> AKIIFIEHNGTRHEVEAKPGLTVMEAARDNGVPGIDADCGGACACSTCHAYVDPAWVDKLPKALPTET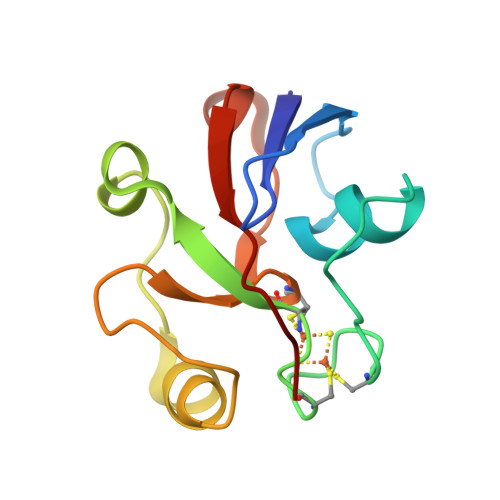DMIDFAYEPNPATSRLTCQIKVTSLLDGLVVHLPEKQI>[2x]MAHHHHHHMLKLIVETKTLVQSLGFASSVVEKRNVIPEYANIKLSAQDGNLELSSTNMDLYLSQKIAVQVVSEGECTVSTKTLNDIVRKLPDSELTLTDLGTTGLEIKGKNCKFNLFTLPVSSFPAMDSINPEASFKISCTDFAKIIESTKFSISLDE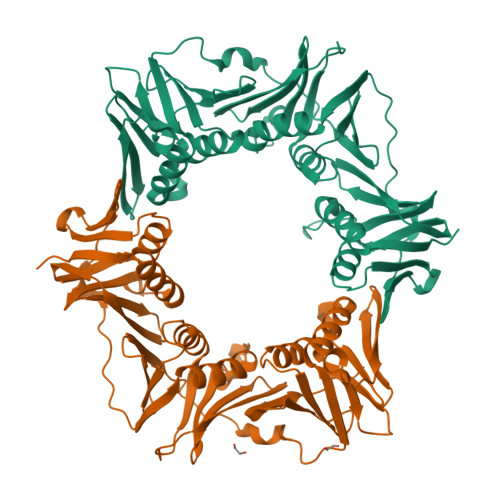TRYNLNGVYLHIKDKEFCSASTDGHRLSISWVTLEKQIKNFGVILPQKSAEEILKIVKDPKNINEDIEILLNSNKIKFICNENTIMLSKLIDGTFPDYSTFIPESSSSKLVINRKMFADSIERIAIITVEKFRAVKLSLSRETLEISAVGEARGNAKEVINSSQDKESFYEYNSDESLAIGFNPQYLEDVLKAVKSDLVELYFSDVSAPVLIKFPENPKDIFVVMPVKV> MGHHHHHHMLTSSSPSQVKTSSEEEWEAASEPDYDTNEDLLYPYSPTPYFGMYHLVKIPIGRGLLHHVDYWGEGKVTNLGKIRGFPQSYNVNEQFALVSKGHNKGKQIPNRIPVVSVDDSDTSSYIRDDSVKTVTISTGPITKRCAADVARIVNASEGLVVAYGYSDNSDDIQNLERELGKKGLYYGAGYELPA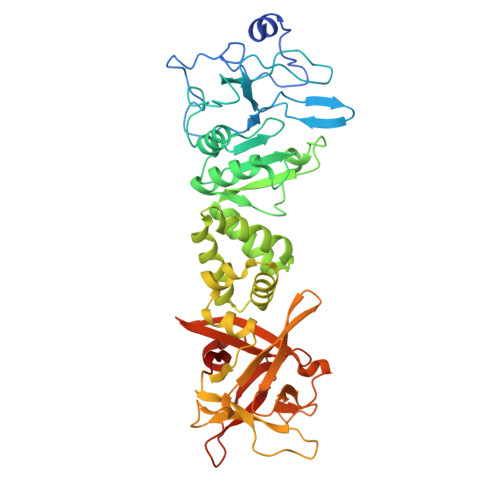DLRTQTEFSTKRVFADASSINNHLYNLVTGGDYINAVKTVRSLVDNQGSDVCRDVVSQLVSHGIKNAMSFAYKLWHEGHKDIVEDYFPSEFQLILDQKRIKLIGKHYNQALKLDANVDRYNDRLTWGDGKDNTSYRVSWRLISLWENNNVIFKILNTEHEMYLKLDVNVDSYGDRKTWGSNDSSEKRHTWYLYPVKVGDQQLFLIENREYRQGLKLDANVDWYGDRLVWGNNGTVADNPEYYGFIIQPWQ In contrast, a group of bacteriophages belonging to families Siphoviridae and Podoviridae has abandoned the usage of one of them, adenine (A), replacing it with 2-aminoadenine (Z). Recently, two classes of replicative proteins found in ZTGC-DNA-containing phages were characterized and one of them, DpoZ from DNA polymerase A (PolA) family, was shown to possess significant Z-vs-A specificity. Phylogenetically speaking, DpoZ are split into two distinct subfamilies: ϕVC8-like and Wayne-like. Both harbour 5′-3′ polymerase and 3′-5′ exonuclease domains and display a strong exonuclease activity. ϕVC8-like DpoZ were studied in detail for phages ϕVC8 and SH-Ab 15497, showing catalytic efficiencies greater by 1–2 orders of magnitude with dZTP than with dATP. The enzyme exhibits the typical fold of the PolA family, with easily identifiable polymerase (pol) and 3′-5′ exonuclease (exo) domains.

Here, we present the crystallographic structure of the apo form of DpoZ of vibriophage ϕVC8, composed of the 3′-5′ exonuclease and polymerase domains. Through extensive screening and optimization, we could eventually obtain single crystals that diffracted to 2.8 Å. The two molecules contained in the asymmetric unit of the DpoZ crystal represent different conformations. The transition between the two forms of the molecule involves mainly two subdomains moving mostly as rigid-bodies: the thumb subdomain known to hold the nascent double-stranded DNA and an extension in the exonuclease domain, present in a reduced form in only a few other PolA structures (see below). Thus, the two DpoZ conformations are hereafter referred to as the ‘thumb-exo’ open and ‘thumb-exo’ closed states. Their RMSD is 2.0 Å for the whole chain, 1.8 Å for the polymerase domain and 1.4 Å for the exonuclease module. Importantly, modelling of the dsDNA substrate in the polymerase domain of DpoZ indicates that the thumb subdomain in its closed state prevents the correct binding of the nucleic acid substrate. The three insertions conserved in the ϕVC8-like DpoZ subfamily take the form of external loops of several to about twenty residues, scattered around the polymerase domain's active site. Indeed, modelling a leaving nucleotide in the exo catalytic site in the thumb-exo open conformation showed that residues R161 and M165 of the helix E2 could contact the nucleobase. Interestingly, although their side-chains are unstructured in the absence of this leaving nucleotide, in the closed state these residues are much closer to the core of the exonuclease domain, assuming a particular conformation which blocks the active site from accepting a nucleotide.

>[2x]MAHHHHHHSAARLMKLDWERTGRRMGFIDLSKYEVWSYDTECTGLQYKVDKVFGFSIATPDGQSGYFDVREQPESLQWLAEQVEPYKGTIVCHNASFDYRMSLHSGIKLPLSQIDDTGIRACCINEHESTIFPWTRGRAGDYSLDYLAKKYVGAQKYAEIYDELAALFGGKATRKTQMPNLYRAPSGLVRKYACPDAELTLELWLEQEELIKKRGLERIVAFERKVMPTLIRTEARGVRVDLDYAEQAIFKMDGVVRENQAKMFALAGREFNPNSPKQVREVFGAKEEGGVWKSRDGTILERTATGNPCLDADALRSMTDPLAAAVLELRSNIKTKDTFLAKHVVEHSVGGRVYPNINQMKGEDGGTGTGRLSYTGPALQQIPSRNKRIAAIIKPAFLPEEGQLWLDSDMASFEVRIFAHLVAAYNPAIAKAYAENPELDLHQWVGDLMGIPRNASYSGQPNAKQMNLGMIFNRGDGAVADSLGMPWEWCEFTDKKGELIRYKKAGREAKSIIAAYHSQIQGVKTLATRAQKIAEERGWIQTAHGRRLRFPNGYKSYKASGILIQATAADENKENWLRIEDALGSDGSMILNTHDSYSMSVDENWKPIWERVKKAVERQTLRVPLLLEFDGVGKNWAEAKGLIDVH Caudovirales, the taxonomic order for the tailed double-stranded DNA bacteriophages, is characterized by the presence of a tail—a host cell attachment organelle that is connected to the genome-containing spherical or elongated capsid via a neck. We describe cryo-EM structures of the neck, the neck-capsid and neck-tail junctions, and capsid of the Agrobacterium phage Milano. The tail to capsid junction involves a symmetry mismatch that is bridged by the neck, and is therefore crucial for the assembly of tailed phage. The extensive network of disulfide bonds within and between neck, collar, capsid and tail provides an exceptional structural stability to Milano.

The 15-fold, 12-fold and 3-fold symmetrized maps of the neck were used to build atomic models of the collar, portal, and neck devoid of capsid (portal + neck 1 + neck 2 + tail terminator + collar), respectively. Namely, the dodecameric portal ring (12 × gp7), which is embedded into the capsid shell, connects sequentially to the dodecameric neck 1 ring (12 × gp14), hexameric neck 2 ring (6 × gp15) and hexameric tail terminator ring (6 × gp18). Besides these conserved common elements, the Milano neck complex possesses a unique, external, sheath-like structure surrounding the neck and consisting of four pentadecameric rings of gp13 (15 × gp13) that we name the collar. In the dodecameric neck 1 assembly, the α-helical and β-sandwich domains of gp14 form the core and peripheral ring, respectively. The core ring connects the neck 2 ring to the portal. The lumen protrusion loops form a diaphragm-like structure that constricts the channel spanning all proteins of the neck and the portal protein. These loops decrease the diameter of the neck lumen from ~30 Å to ~18 Å. There are two alternating conformations of the lumen protrusion loop, with six tilted up and six tilted down. The lumen of portal, neck 1, and neck 2 possesses a positive electrostatic potential resulting in a positive charge of the neck lumen —suitable to hold and position the end of the negatively charged linear dsDNA until the genome release.

>MYFFSVDPRNGASKSGDVCGSCCCESISARPGEVNGVMVSYAAWSAPLRGHGLTNKTTFEIDGVSVTPPKVSNAFGRTKVGVVFEGTLSDLFPNPEGEQVEYEISELNGPSNGVVELGANGAFTYTPGALFTGVDRFWFSINGNIGEYVISVDPTTSELPQPPFTTPVYVPAARRSVDPRTHVLKFVLGVSPAAIPGDVYRLTVRQVAIDCDGNEFVHISCYDISIGSCG[60x];>[12x]MLGIPLLTRKAALTPPAPSANPAKIFIRRFFSAGVAKNVVSYSNVMAAQRAMEHPVAFRCLDKLGLTVQSVKWDVGKDPQNTQVGDGGMSASQRKALQQILQRPNPTMSGAQLRYSAALSWACFGRMAFKVSVMSDGSVNAIWPLGIPFLKQKFDRYGDVESFQYGDEAGKETIPSFTKVEKNDKGRPIKNYAFMIVKPSINGAMNFDVQNTPLQAIGVPVALYDALMARAIDSADGTPNSKWLVTASRDLDDGQAKEVKEGIEETKPGGDNGGEIIFIAGTDVKVQEMKNDLSDIHSKVPLDDQARTIAGNFGIPIALLGFAGADGSKFANNYDESRKAFFEDTIEPGYLTPLEDGFSMFLCGAGYRVIFDRDSIPALRKSRADIAATYDKVTFITEEEKREVTGWPAKKEGQTQNDDA;>[6x]MRTADRKHRVIVCSQQSDVDDEGRLLITRAGVIQGWAAIAPVKAIRFSQDGVSMQKDTMQPTHDITMNYNPDVNVSVSAWVYEHRLKSPPRWFKVLSVVNVDECSRYMKIRCRLVETSDDVTPPVEEEKNSFGAVKIDIPL;>METKLTYGNRVTLPEFAKYIVAPAFHEIEGRAIPVTGVDDDASGTQATKLPFVLVGLRQGDTSGPATIAGNSTINLRDDFIVEFNMKKERYRDRKGGETPFFSYYDYESIRDRLFNSMIEFSGEHGITFEFVSLDISTEGDVVYIEFRFRQNYEWCETVREADTTIEAGRFSINLQGC[6x];>[6x]MACNKQNGVKNILITFTDCDTQEVIGPISHEQPDDTLPTYKNCAWTNTALTNGYVQRSASNATMTLPVVRDLRVPLAFYQGCAQVDVQVEKFDGTVMTLTEGAVVEPEESDGRSVTMNIVASEIDELLPPGSLAAA;>[12x]MNLDTLLPLQTIREHAKCDDNPRVTDDLLKLYREAAFEAAELYTGLSFTPEKTIVEPIRLKGRRGKIILSATPIAGRPVVFYGGGLGSPLELIPRPGSNVLFFPYGSPDRFQTWGDCHTCDVESQLMATYVTGRRCENSVPAGIIIGILKLIAWNINNPGDEVMSVRNTLNANAQGLIGGTNNGAVISGAQDEWFRYRRVLL> MYKEPFGVKVDFETGIIEGAKKSVRRLSDMEGYFVDERAWKELVEKEDPVVYEVYAVEQEEKEGDLNFATTVLYPGKVGKEFFFTKGHFHAKLDRAEVYVALKGKG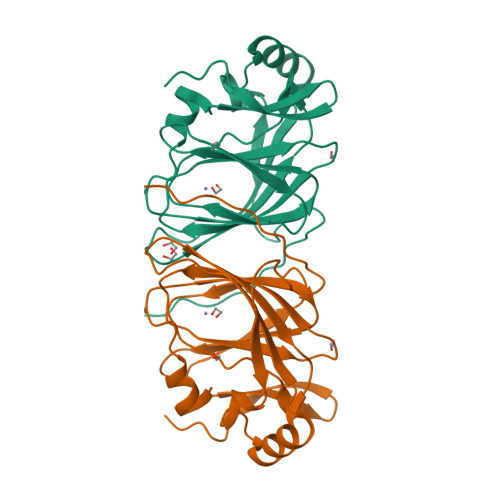GMLLQTPEGDAKWISMEPGTVVYVPAGWAHRTVNIGDEPFIFLAIYPADAGHDYGTIAEKGFSKIVIEENGEVKVVDNPRWKK methyl 9-S-acetyl-5-acetamido-3,5-dideoxy-9-thio-D-glycero-alpha-D-galacto-non-2-ulopyranosidonic acid | C14 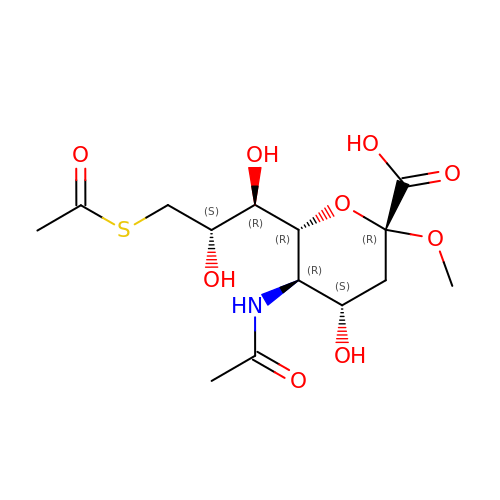H23 N O9 S | QHXQSHGOUBTADZ-KXEMTNKZSA-N>SAMKRRRCGVCEVCQQPECGKCKACKDMVKFGGTGRSKQACLKRRCPNLAVKEADDDEEADDDVSEMPSPKKLHQGKKKKQNKDRISWLGQPMKIEENRTYYQKVSIDEEMLEVGDCVSVIPDDSSKPLYLARVTALWEDKNGQMMFHAHWFCAGTDTVLGATSDPLELFLVGECENMQLSYIHSKVKVIYKAPSENWAMEGGTDPETTLPGAEDGKTYFFQLWYNQEYARFESPPKTQPTEDNKHKFCLSCIRLAELRQKEMPKVLEQIEEVDGRVYCSSITKNGVVYRLGDSVYLPPEAFTFNIKVASPVKRPKKDPVNETLYPEHYRKYSDYIKGSNLDAPEPYRIGRIKEIHCGKKKGKVNEADIKLRLYKFYRPENTHRSYNGSYHTDINMLYWSDEEAVVNFSDVQGRCTVEYGEDLLESIQDYSQGGPDRFYFLEAYNSKTKNFEDPPNHARSPGNKGKGKGKGKGKGKHQVSEPKEPEAAIKLPKLRTLDVFSGCGGLSEGFHQAGISETLWAIEMWDPAAQAFRLNNPGTTVFTEDCNVLLKLVMAGEVTNSLGQRLPQKGDVEMLCGGPPCQGFSGMNRFNSRTYSKFKNSLVVSFLSYCDYYRPRFFLLENVRNFVSYRRSMVLKLTLRCLVRMGYQCTFGVLQAGQYGVAQTRRRAIILAAAPGEKLPLFPEPLHVFAPRACQLSVVVDDKKFVSNITRLSSGPFRTITVRDTMSDLPEIQNGASNSEIPYNGEPLSWFQRQLRGSHYQPILRDHICKDMSPLVAARMRHIPLFPGSDWRDLP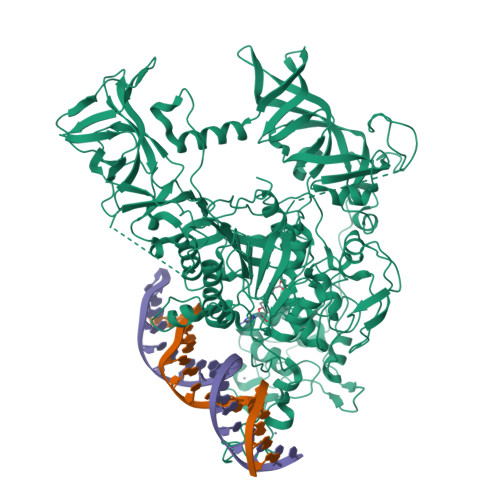NIQVRLGDGVIAHKLQYTFHDVKNGYSSTGALRGVCSCAEGKACDPESRQFSTLIPWCLPHTGNRHNHWAGLYGRLEWDGFFSTTVTNPEPMGKQGRVLHPEQHRVVSVRECARSQGFPDSYRFFGNILDRHRQVGNAVPPPLAKAIGLEIKLCLLSSA[2x]>[2x]AEMPKRKFTIDDFDIVRPLGKGKFGNVYLAREKQNKFIMALKVLFKSQLEKEGVEHQLRREIEIQSHLRHPNILR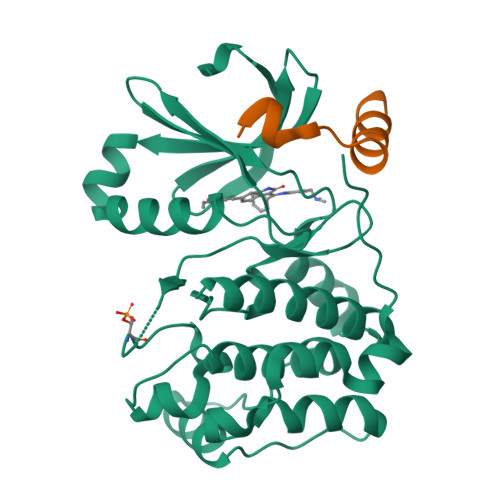MYNYFHDRKRIYLMLEFAPRGELYKELQKHGRFDEQRSATFMEELADALHYCHERKVIHRDIKPENLLMGYKGELKIADFGWSVHAPSLRRRTMCGTLDYLPPEMIEGKTHDEKVDLWCAGVLCYEFLVGMPPFDSPSHTETHRRIVNVDLKFPPFLSDGSKDLISKLLRYHPPQRLPLKGVMEHPWVKANSRRVLPPVYQ;>[2x]MDESQPRKPIPAWASGNLLTQAIRQQYYKPIDVDRMYGTIDSPKLEELFNKSKPRYFKR>MNHKVHHHHHHIEGRHMTNTRSAVVLGGGMAGMLVSSMLARHVGSVTVIDRDAFPAGPDLRKGVPQARHAHILWSGGARIVEELLPGTTDRLLGAGAHRIGIPDGQVSYTAYGWQHRFPEAQFMIACSRALLDWTVREETLREERIALVEKTEVLALLGDAGRVTGVRVRDQESGEEREVPADLVVDTTGRGSPMKRLLAELGLPAPEEEFVDSGMVYATRLFRAPEAAATNFPLVSVHADHRAGRPGCNAVLMPIEDGRWIVTVSGTRGGEPPADDEGFARFARDGVRHPLVGELIAXAQPLTSVERSRSTVNRRLHYDRLATWPEGLVVLGDAVAAFNPVYGHGMSAAAHSVLALRSQLGQRAFQPGLARAAQRAIAVAVDDAWVLATSHDIGYPGCRTQTRDPRLTRHAGERQRVTDLVGLTATRNQVVNRAAVALNTLSAGMASMQDPAVMAAVRRGPEVPAPTEPPLRPDEVARLVSGAGVTA[2x]

Lasalocid A, a polyether ionophore natural product derived from Streptomyces lasalocidi, is a widely used veterinary medicine that acts by transporting various cations across the cell membrane, thereby disrupting cation homeostasis. Lasalocid A biosynthesis entails two stereospecific epoxidation of the precursor diene, catalyzed by the flavin-dependent enzyme Lsd18. We performed protein engineering on Lsd18 to improve its thermostability and catalytic activity. Screening of these mutants using thermal shift assay identified stabilized variants Lsd18-T189M, Lsd18-S195M, and the double mutant Lsd18-T189M-S195M.

We found that the Tm values of Lsd18-T189M, Lsd18-S195M, and Lsd18-T189M-S195M were increased by 3.0 °C, 4.5 °C, and 4.8 °C, respectively. After incubating these proteins with trypsin for 45 min, the wild-type Lsd18 completely disappeared, while some intact proteins remained for the three mutants, especially for Lsd18-S195M and Lsd18-T189M-S195M. The stability of the system is obviously improved by the S195M mutation, and the captured structure is almost stable in one conformation. In order to reveal the structural basis for the higher thermostability of the best two mutants, we solved the crystal structures of Lsd18-S195M and Lsd18-T189M-S195M at the resolution of 2.50 Å and 3.76 Å, respectively. Comparing the structures of Lsd18 WT, Lsd18-S195M, and Lsd18-T189M-S195M, it can be seen that the angle of the α helix between L408 and T419 shifts, which is in agreement with the MD study. However, in the crystal structure of Lsd18-S195M, a loop in this region turns to a helix, indicating the effect of stabilization. Furthermore, the loop region R314-L316, E208-F210 and C398-Q401 in Lsd18 WT change to a β sheet in the two mutants’ crystal structures, also indicating that this region is less flexible and more stable. In wild-type Lsd18, there is a hydrogen bonding network between S195 and D187, S193 and L199. Moreover, weak hydrogen bonds formed between S195 and L198, as well as Y319. After mutating from S195 to M195, the hydrogen bonds involving D187 and Y319 were removed and new hydrophobic interactions formed between M195 and L199, as well as V331.>MKITVVDLGNINVKYVGENKGRFSSKITNDYQSYEEGFQRVEYNGIKTYIGVGELSREFNKADRDYMAQLLYSLAKANTADTKEINLTLLLPIIQMKNKTRLIETLKGENFKFKFNGIDREIKINDLMVLPEGYASYYSLDIENKKGDVCILDLGSRTINICVLENAKIVKTNTIKLGSFDFYSKIKSLENAKGEDYIEEDIQRLIDNGLIKVDSKQYIEFLSDILNAVKPYVNLKTYNTIFTGGTSLMLKEYIEKLP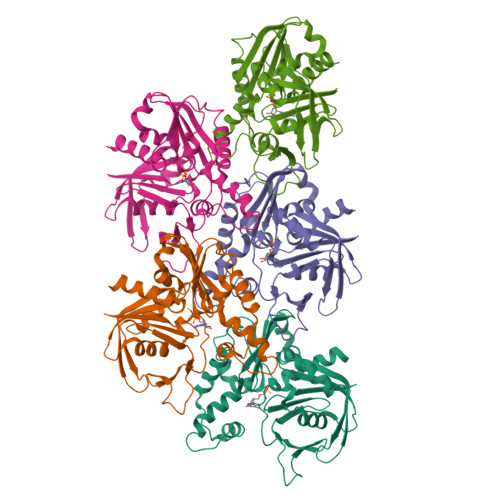LNKFKVHPNALTSNVDGAMEASKKVWN[5x]>STAGKVIKCKAAVLWEEKKPFSIEEVEVAPPKAHEVRIKMVATGIC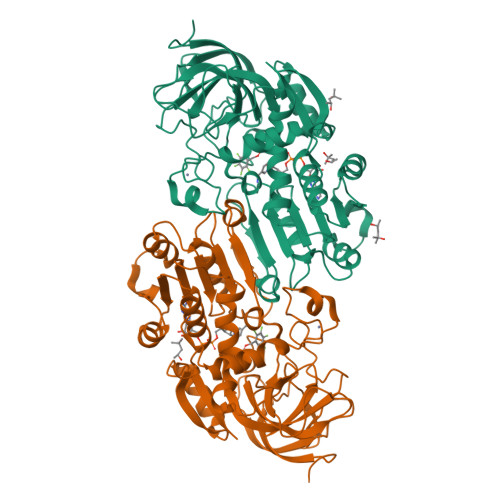RSDDHVVSGTLVTPLPVIAGHEAAGIVESIGEGVTTVRPGDKVIPLFTPQCGKCRVCKHPEGNFCLKNDLSMPRGTMQDGTSRFTCRGKPIHHFLGTSTFSQYTVVDEISVAKIDAASPLEKVCLIACGFSTGYGSAVKVAKVTQGSTCAVFGLGGVGLSVIMGCKAAGAARIIGVDINKDKFAKAKEVGATECVNPQDYKKPIQEVLTEMSNGGVDFSFEVIGRLDTMVTALSCCQEAYGVSVIVGVPPDSQNLSMNPMLLLSGRTWKGAIFGGFKSKDSVPKLVADFMAKKFALDPLITHVLPFEKINEGFDLLRSGESIRTILTF[2x]>SPVEWTVMDVVEYFTEAGFPEQATAFQEQEIDGKSLLLMQRTDVLTGLSIRLGPALKIYEHHI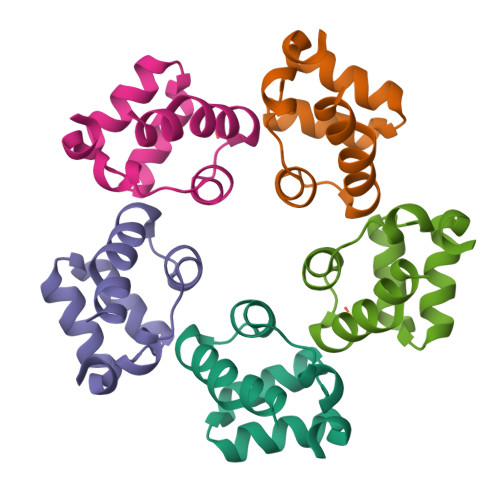KVLQQG[20x]5-azanyl-3-[1-(pyridin-3-ylmethyl)indol-6-yl]-1~{H}-pyrazole-4-carbonitrile 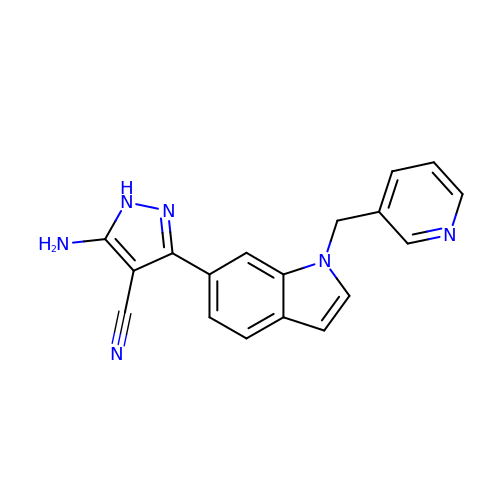| C18 H14 N6 | LBFCIYHKVAYEJG-UHFFFAOYSA-N> EPIRYAIPEELDRGSLVGNLAKDLGFGVGDLPTRNLRVIAEKKFFTVSPENGNLLVSDRIDREEICGKKSTCVLEFEMVAEKPLNFFHVTVLIQDINDNPPTFSQNITELEISELALTGATFALESAQDPDVGVNSLQQYYLSPDPHFSLIQKENLDGSRYPELVLKAPLDREEQPHHHLVLTAVDGGEPSRSCTTQIRVIVADANDNPPVFTQDMYRVNVAENLPAGSSVLKVMAIDMDEGINAEIIYAFINIGKEVRQLFKLDSKTGELTTIGELDFEERDSYTIGVEAKDGGHHTAYCKVQIDISDENDNAPEITLASESQHIQEDAELGTAVALIKTHDLDSGFNGEILCQLKGNFPFKIVQDTKNTYRLVTDGALDREQIPEYNVTITATDKGNPPLSSSKT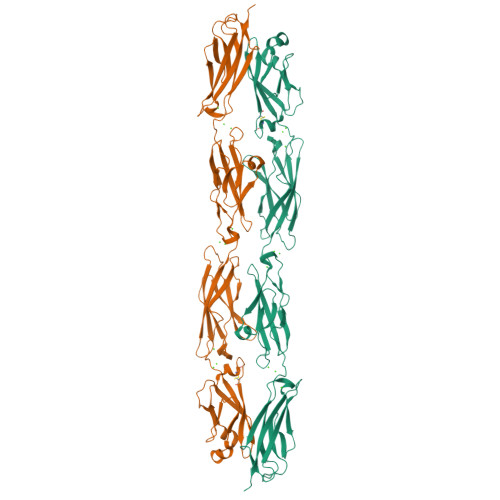ITLHILDAA>[8x]SNAQGPPLPLNQGQLLPLAQGLPLAVSPALPSNPTD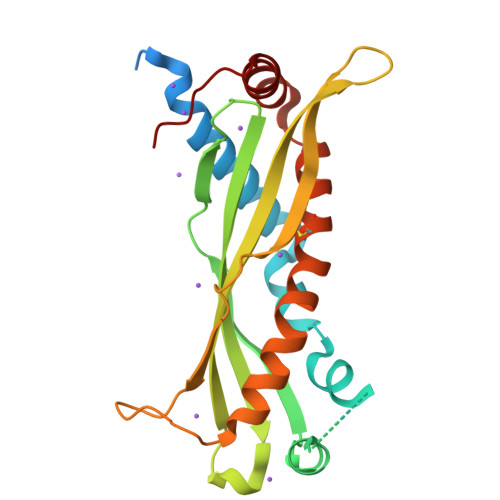LLAGKFTDALSGGLLSGGLLGILENIPLLDVIKSGGGNSNGLVGGLLGKLTSSVPLLNNILDIKITDPQLLELGLVQSPDGHRLYVTIPLGLTLNVNMPVVGSLLQLAVKLNITAEVLAVKDNQGRIHLVLGDCTHSPGSLKISLLNGVTPVQSFLDNLTGILTKVLPELIQGKVCPLVNGILSGLDVTLVHNIAELLIHGLQFVIKV>[6x]MEFKKVAKETAITLQSYLTYQAVRLISQQLSETNPGQAIWLGEFSKRHPIQESDLYLEAMMLENKELVLRILTVRENLAEGVLEFLPEMVLSQIKQSNGNHRRSLLER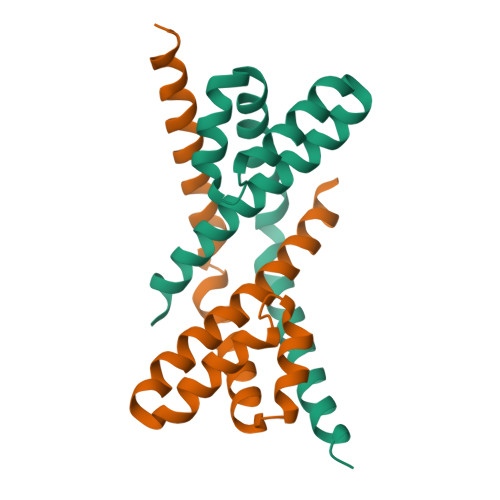LTQVDSSSTDQTEPNPGESDTSEDSE> ETIEII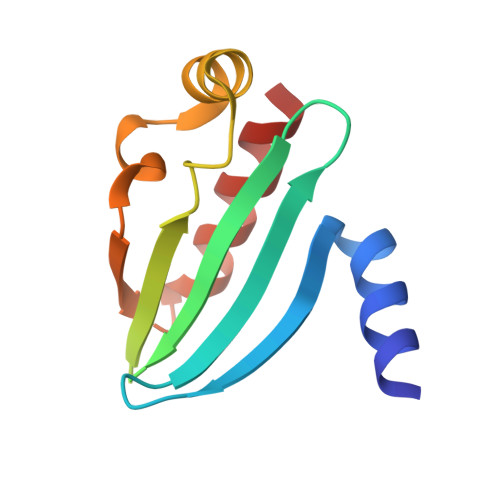KDLFEHLCGVRVHRTYEDDTGLWFDTSQGSKNGIMDYKLGFVKSQAENTTEVDTEVIYVPLLKQRTAEELQELQKKLPDYLFETLSFPLRSLNQFYIKMSKSLNKKV> MKLDIKKTFSNRSDRVKGIDFHPTEPWVLTTLYSGRVELWNYETQVEVRSIQVTETPVRAGKFIARKNWIIVGSDDFRIRVFNYNTGEKVVDFEAHPDYIRSIAVHPTKPYVLSGSDDLTVKLWNWENNWALEQTFEGHEHFVMCVAFNPKDPSTFASGCLDRTVKVWSLGQSTPNFTLTTGQE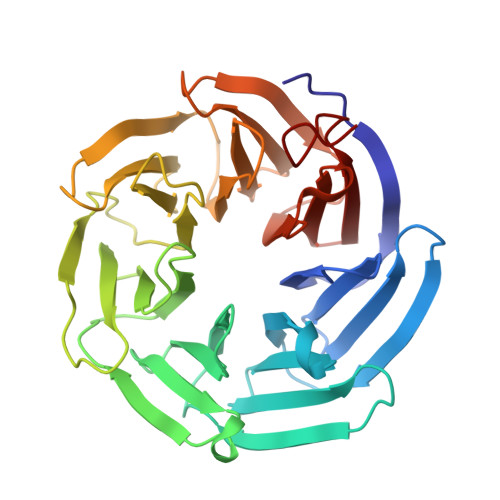RGVNYVDYYPLPDKPYMITASDDLTIKIWDYQTKSCVATLEGHMSNVSFAVFHPTLPIIISGSEDGTLKIWNSSTYKVEKTLNVGLERSWCIATHPTGRKNYIASGFDNGFTVLSLGNDEHHHHHH>[4x]FEEEDVICDGCNGPVVGTRYKCSVCPDYDLCSVCEGKGLHRGHTKLAFPSPFGHLSEGFS

Intriguingly, the autophagy adapter p62/SQSTM1/Sequestosome-1 was recently reported to recognize N-degrons, the N-end rule substrates of the well-characterized UPS, and where ultimately these substrates are delivered to ALS8,9. p62 is a key selective autophagy adapter that plays a role in the degradation of various cellular constituents such as misfolded proteins and their aggregates, malfunctioning organelles, and invading pathogens. Intriguingly, it was recently reported that the central ZZ-domain in p62 plays a critical role in the recognition of N-terminal arginylated BiP/GRP78 by the Arg-tRNA transferase ATE1. Here, we present the high resolution structures of the ZZ-domain of p62 in complex with 8 different N-degrons including type-1 and type-2, and subsequently identify key determinants involved in the unusual recognition.

However, an understanding of the manner by which the ZZ-domain binds to type-2 substrates is problematic since there is no deep hydrophobic pocket in the ZZ-domain, which is known to be involved in the recognition mode for type-2 N-degrons. Therefore, we determined the structure of the ZZ-domain in complex with a variety of N-degrons comprising three type-1 N-degrons and five type-2 N-degrons. As described for the R-BiP complex, two aspartic acid residues, Asp129 and Asp149, bind to the α-amino group, and Asp147 forms a hydrogen bond with the first peptide bond, which means that these interactions are conserved in all different N-terminal residues. However, the side chain of the N-terminal residue of the N-degron is recognized differently. Furthermore, the hydrophobic side chain of Ile127 guides the orientation of the side chain of the primary residue. Furthermore, the phenyl ring of the phenylalanyl peptide is properly oriented for van der Waals interactions. Our structural information clearly explains the affinity measurement data as well as previous pull-down assay results showing that type-1 N-degrons and only a subset of type-2 N-degron peptides (Phe, Trp, and Tyr) displayed binding affinity with p62.>[5x]MSLLSDLCNLNLSESTEKIIAEYIWIGGSGMDLRSKARTLNAPVSDPSKLPQWNYDGSSTGQAPGEDSEVILYPQAIYKDPFRRGNNILVMCDAYTPGGEPIPTNKRFDAAKIFSHPDVVAEEPWYGIEQEYTLLQKEVKWPIGWPVGGYPGPQGPYYCGIGADKAFGRDI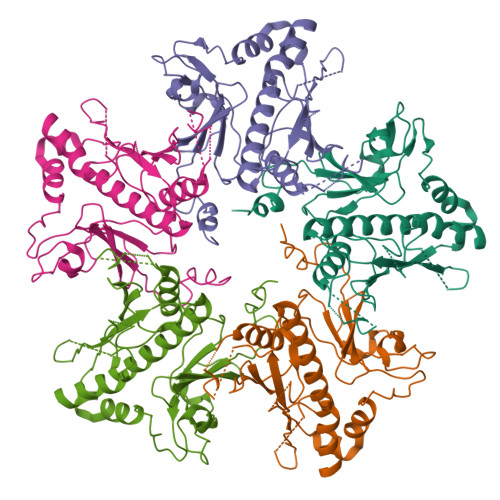VDAHYKACLYAGINISGINGEVMPGQWEFQVGPSVGISSGDQLWMARYILERITEIAGVVVSFDPKPIEGDWNGAGAHTNYSTKSMRSDGGFEVIKKAIEKLGLKHREHIAAYGEGNERRLTGKHETADINTFLWGVANRGASIRVGRDTEKAGKGYFEDRRPASNMDPYIVTSMIANTTILWKP> XTSFK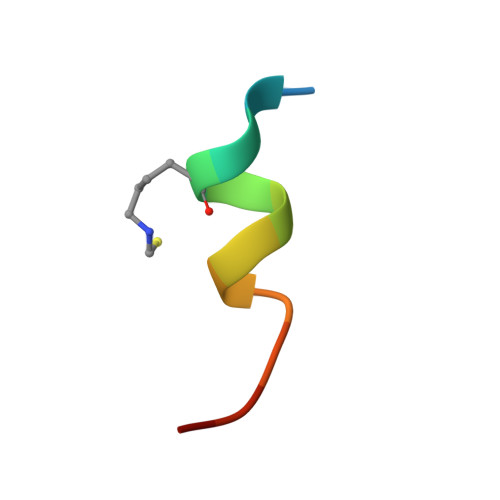EYWCLLSPX> GDVEEAIDRAVARVADTMPTGPRNTESVPALTAVETGHTSQVVPGDTMQTRHVKNYHSRTESSIENFLCRAACVYIATYKSAGGTPTERYASWRINTRQMVQLRRKFELFTYLRFDMEITFVITSTQDPGTQLAQDMPVLTHQIMYIPPGGPVPNSATDFAWQSSTNPSIFWTEGCAPARMSVPFISIGNAYSNFYDGWSHFTQEGVYGFNSLNNMGHIYVRHVNEQSLGVSTSTLRVYFKPKHVRAWVPRPPRLSPYVKSSNVNFKPTAVTT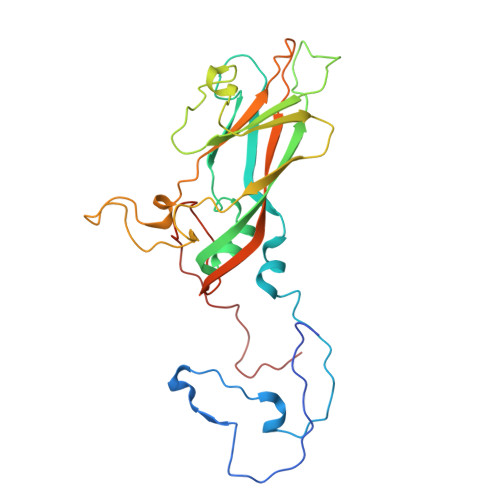ERKDINDVGT>[4x]AKRKRIEMYTKASFKASNQKIEQIWKTQQEEIQKLNNEYSQQFMNVLQQWELDIQKFEEQGEKLSNLFRQQQKIFQQSRIVQ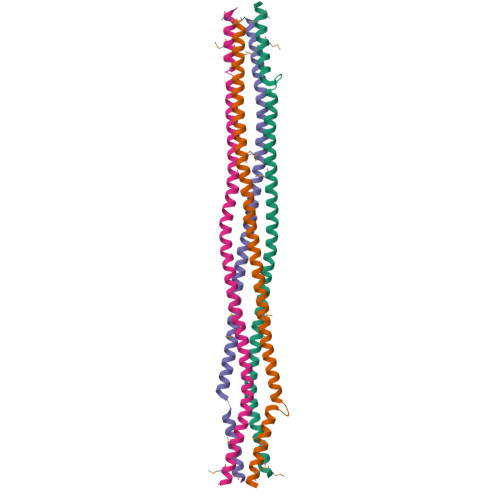SQRMKAIKQIHEQFIKSLEDVEKNNDNLFTGTQSELKKEMAMLQKKVMMETQQQEMANVRKS>[2x]ETKFVQALFDFNPQESGELAFKRGDVITLINKDDPNWWEGQLNNRRGIFPS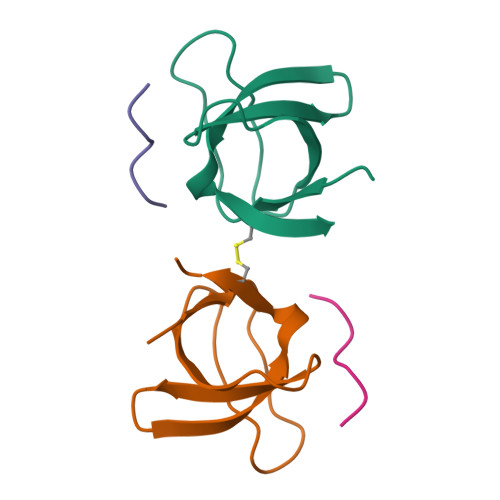NYVCPYN;>[2x]XPPPVPPRRR>[2x]VLDGPYQPTSFNLP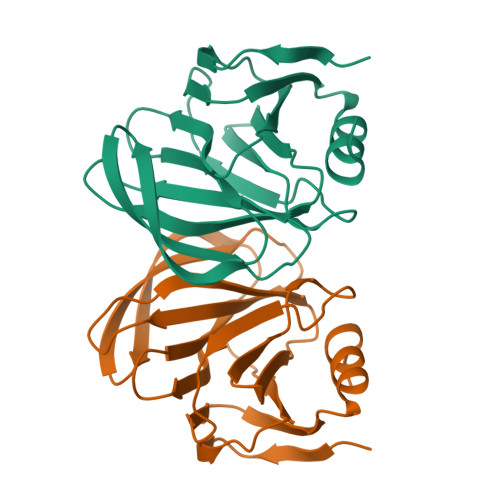VDYWMMMSPTQAGRVAEGTNGTDRWFACIIVEPNVSLQSRDYVLDGQTVQLQVDNTSNTMWKFILFIKLTKSGNYSQYSSLLTNHKLCAWIKRDSRVYWFDGTVPNSSDNYYLTINNDNSIVSSDVDFYLIPRTQTDSCRRCINNGL> LDFSKWKTRQPGEFRAPCPAMNSLANHGFIPRDGRNITVAMLVPVLQEVFHLSPELAQTISTLGLFTAQDPSKGVFTLDDLNRHNLFEHDASLSREDYYFHKDASTFRPEVFKKFMSHFKGKEYVTLEDAASARYAMVQESRKKNPTFTYTVQQRITSYGETIKYFRTIVEPATGKCPVAWIKILFEQERLPYNEGWRPPKAE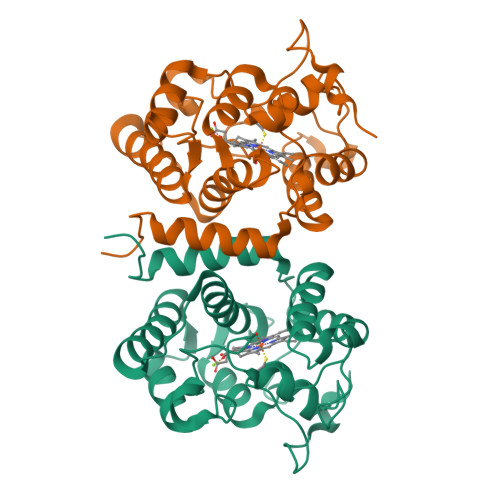LSGFSMASDVLELALVTPEKLID;> ALDFSKWKTRQPGEFRAPCPAMNSLANHGFIPRDGRNITVAMLVPVLQEVFHLSPELAQTISTLGLFTAQDPSKGVFTLDDLNRHNLFEHDASLSREDYYFHKDASTFRPEVFKKFMSHFKGKEYVTLEDAASARYAMVQESRKKNPTFTYTVQQRITSYGETIKYFRTIVEPATGKCPVAWIKILFEQERLPYNEGWRPPKAELSGFSMASDVLELALVTPEKLID> GTLDSTWKEATLPQVKAMLEKDDGKVSGDTVTYSGKTVHVVAAAVLPGFPFPSFEVHDKKNPTLEIPAGATVDVTFINTNKGFGHSFDITKKGPPYAV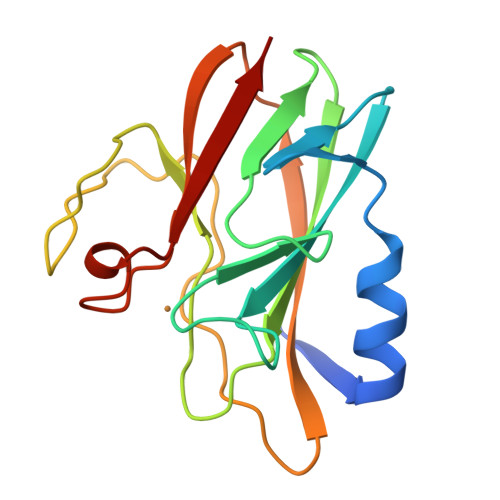MPVIDPIVAGTGFSPVPKDGKFGYTDFTWHPTAGTYYYVCQIPGHAATGMFGKIVVK9-METHYLGUANINE | C6 H7 N5 O | 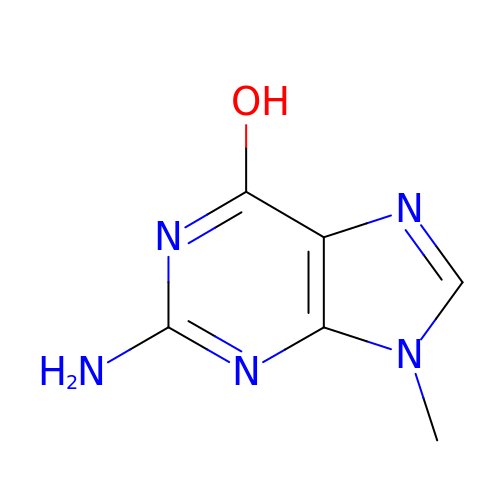UUWJNBOCAPUTBK-UHFFFAOYSA-N Vertebrate type-IIa RPTPs comprise LAR, PTPσ and PTPδ, which share common domain architecture with a single transmembrane (TM) helix flanked by a large extracellular domain (ECD) and cytoplasmic tandem PTP domains: the membrane-proximal PTP domain (D1) is catalytically active, whereas the membrane-distal PTP domain (D2) is inactive. In mammals, presynaptic type-IIa RPTPs form trans-synaptic adhesion by specifically binding to their cognate postsynaptic organizers through their ECDs for inducing synaptic differentiation of neurons. To date, five different types of postsynaptic organizers for type-IIa RPTPs have been reported: interleukin-1 receptor (IL-1R) accessory protein (IL-1RAcP)7, IL-1RAcP-like-1 (IL1RAPL1)8, neurotrophin receptor tyrosine kinase C (TrkC), netrin-G ligand-3 (NGL-3)1011 and Slit- and Trk-like (Slitrk) family proteins. To elucidate the structural basis for decoding the ‘splice-insert signaling code' in the type-IIa RPTPs, we determined the crystal structures of PTPδ-ECD in complex with IL-1RAcP-ECD and IL1RAPL1-ECD.

To elucidate the structural basis of the PTPδ–IL1RAPL1 interaction for trans-synaptic adhesion, we determined the crystal structures of IL1RAPL1-ECD in complex with PTPδ Ig1-Ig2 and the full-length PTPδ-ECD at 2.7 and 4.4 Å resolutions, respectively. For crystallography, we used a PTPδ isoform containing four Fn domains and both meA9 and meB, which is the most abundant in the developing brain and has the highest affinity for IL1RAPL1 (Kd: 0.15 μM) among all the PTPδ variants. PTPδ-ECD binds to IL1RAPL1-ECD at a ratio of 1:1 and the asymmetric unit contains one PTPδIL1RAPL1 complex. PTPδ-ECD exhibits an elongated shape with a length of 180 Å along the longest axis. The Ig3 domain is spatially separated by the meB-containing linker and positioned apart from the Ig1-Ig2 unit. The Fn3 domain of PTPδ is oriented perpendicular to the Fn1-Fn2 domains, as observed in the PTPσ Ig1-Fn3 structure. Electron density of the Fn4 domain and subsequent C-terminal region was not visible, likely due to the disorder. The length of the PTPδ-ECD·IL1RAPL1-ECD complex along the longest axis is 206 Å, which is equivalent to the average length of excitatory synaptic clefts, implying that PTPδ-ECD is kinked at the junction between the Fn2 and Fn3 domains in synapses. On the opposite side to the IL1RAPL1 Ig1–PTPδ Ig2 interface, the Ig1 domain of IL1RAPL1 interacts with the Ig3 domain of PTPδ with a buried surface area of 694 Å2. In the present PTPδ-ECDIL1RAPL1-ECD complex, the meB insertion appears to adjust the relative spacing and orientation between the Ig2 and Ig3 domains of PTPδ.

> ETPPRFTRTPVDQTGVSGGVASFICQATGDPRPKIVWNKKGKKVSNQRFEVIEFDDGSGSVLRIQPLRTPRDEAIYECVASNNVGEISVSTRLTVLREDQIPRGFPTIDMGPQLKVVERTRTATMLCAASGNPDPEITWFKDFLPVDTSNNNGRIKQLRSESIGGTPIRGALQIEQSEESDQGKYECVATNSAGTRYSAPANLYVRELREVRRVPPRFSIPPTNHEIMPGGSVNITCVAVGSPMPYVKWMLGAEDLTPEDDMPIGRNVLELNDVRQSANYTCVAMSTLGVIEAIAQITVKALPKPPGTPVVTESTATSITLTWDSGNPEPVSYYIIQHKPKNSEEPYKEIDGIATTRYSVAGLSPYSDYEFRVVAVNNIGRGPASEPVLTQTSEQAPSSAPRDVQARMLSSTTILVQWKEPEEPNGQIQGYRVYYTMDPTQHVNNWMKHNVADSQITTIGNLVPQKTYSVKVLAFTSIGDGPLSSDIQVITQTGVPGQPLNFKAEPESETSILLSWTPPRSDTIASYELVYRDGDQGEEQRITIEPGTSYRLQGLKPNSLYYFRLSARSPQGLGASTAEISARTMQSMFAKNFHVKAVMKTSVLLSWEIPENYNSAMPFKILYDDGKMVEEVDGRATQKLIVNLKPEKSYSFVLTNRGNSAGGLQHRVTAKTAPDVLRTKPAFIGKTNLDGMITVQLPDVPANENIKGYYIIIVPLKKSRGKFIKPWESPDEMELDELLKEISRKRRSIRYGREVELKPYIAAHFDVLPTEFTLGDDKHYGGFTNKQLQSGQEYVFFVLAVMDHAESKMYATSPYSDPVVSMDLDPQPITDEEEKHHHHHH;> AQPAARDLKVVTKRGSADGCTDWSVDIKKYQVLVGEPVRIKCALFYGYIRTNYSLAQSAGLSLMWYKSSGPGDFEEPIAFDGSRMSKEEDSIWFRPTLLQDSGLYACVIRNSTYCMKVSISLTVGENDTGLCYNSKMKYFEKAELSKSKEISCRDIEDFLLPTREPEILWYKECRTKAWRPSIVFKRDTLLIKEVKEDDIGNYTCELKYGGFVVRRTTELTVTAPLTDKPPKLLYPMESKLTVQETQLGGSANLTCRAFFGYSGDVSPLIYWMKGEKFIEDLDENRVWESDIRILKEHLGEQEVSISLIVDSVEEGDLGNYSCYVENGNGRRHASVLLHKRKHHHHHH>MTTAGVSRRPGRLAGKAAIVTGAAGGIGRATVEAYLREGASVVAMDLAPRLAATRYEEPGAIPIACDLADRAAIDAAMADAVARLGGLDILVAGGALKGGTGNFLDLSDADWDRYVDVNMTGTFLTCRAGARAMVAAGAGKDGRSARIITIGSVNSFMAEPEAAAYVAAKGGVAMLTRAMAVDLARHGILVNMIAPGPVDVTGNNTG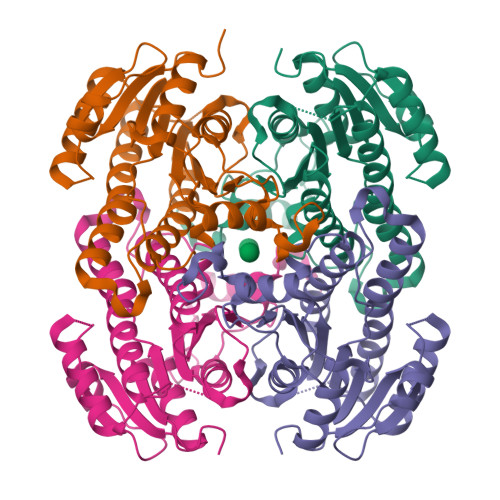YSEPRLAEQVLDEVALGRPGLPEEVATAAVFLAEDGSSFITGSTITIDGGLSAMIFGGMREGRR[4x]>[4x]IGVASFAKAFPWHFI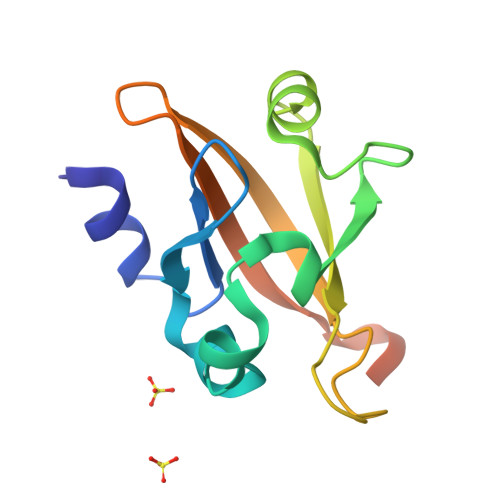TDKRLELVQLGAGFMRLFGTHLATHGSSLGTYFRLLRPRGVPLDFREILKRVNTPFMFALKMPGSTALAEGLEIKGQMVFAAESDSLLFVGSPFLDGLEGLTGRGLFISDI>[13x]MGSSHHHHHHSQDLDEVDAGSMTEIVA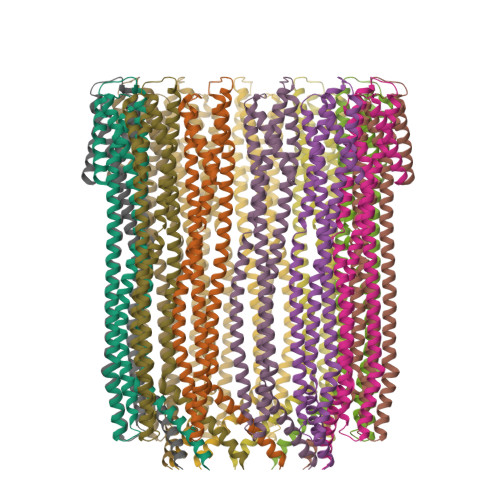DKTVEVVKNAIETADGALDLYNKYLDQVIPWQTFDETIKELSRFKQEYSQAASVLVGDIKTLLMDSQDKYFEATQTVYEWCGVATQLLAAYILLFDEYNEKKASAQKDILIKVLDDGITKLNEAQKSLLVSSQSFNNASGKLLALDSQLTNDFSEKSSYFQSQVDKIRKEAYAGAAAGVVAGPFGLIISYSIAAGVVEGKLIPELKNKLKSVQNFFTTLSNTVKQANKDIDAAKLKLTTEIVAIGEIKTETETTRFYVDYDDLMLSLLKEAAKKMINTCNEYQKRHGKKTLFEVPEV>MTQFNPVDHPHRRYNPLTGQWILVSPHRAKRPWQGAQETPAKQVLPAHDPDCFLCAGNVRVTGDKNPDYTGTYVFTNDFAALMSDTPDAPESHDPLMRCQSARGTSRVICFSPDHSKTLPELSVAALTEIVKTWQEQTAELGKTYPWVQVFENKGAAMGCSNPHPHGQIWANSFLPNEAEREDRLQKEYFAEQKSPMLVDYVQRELADGSRTVVETEHWLAVVPYWAAWPFETLLLPKAHVLRITDLTDAQRSDLALALKKLTSRYDNLFQCSFPYSMGWHGAPFNGEENQHWQLHA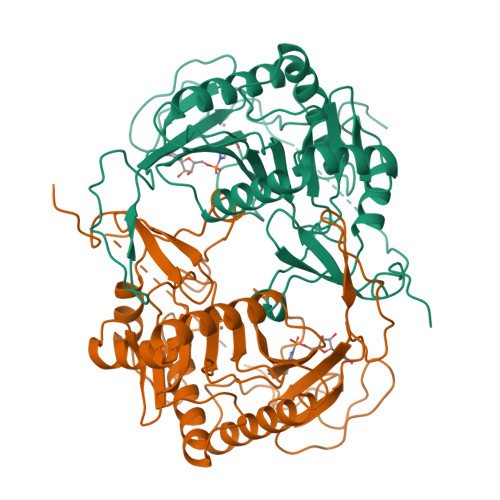HFYPPLLRSATVRKFMVGYEMLAETQRDLTAEQAAERLRAVSDIHFRESGV[2x]>[2x]MATATEQWVLVEMVQALYEAPAYHLILEGILILWIIRLLFSKTYKLQERSDLTVKEKEELIEEWQPEPLVPPVPKDHPALNYNIVSGPPSHKTVVNGKECINFASFNFLGLLDNPRVKAAALASLKKYGVGTCGPRGFYGTFDVHLDLEDRLAKFMKTEEAIIYSYGFATIASAIPAYSKRGDIVFVDRAACFAIQKGLQASRSDIKLFKHNDMADLERLLKEQEIEDQKNPRKARVTRRFIVVEGLYMNTGTICPLPELVKLKYKYKARIFLEESLSFGVLGEHGRGVTEHYGINIDDIDLISANMENALASIGGFCCGRSFVIDHQRLSGQGYCFSASLPPLLAAAAIEALNIMEENPGIFAVLKEKCGQIHKALQGISGLKVVGESLSPAFHLQLEESTGSREQDVRLLQEIVDQCMNRSIALTQARYLEKEEKCLPPPSIRVVVTVEQTEEELERAASTIKEVAQAVLL;>MRPEPGGCCCRRTVR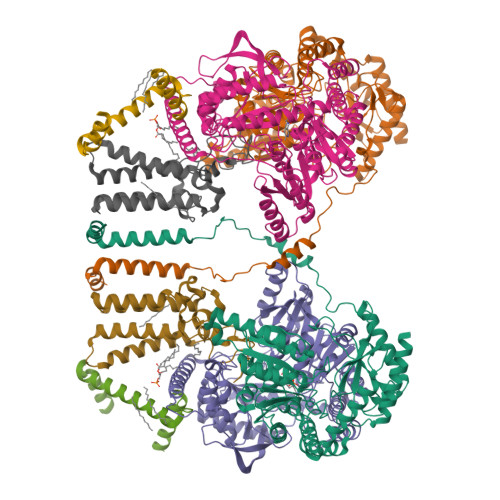ANGCVANGEVRNGYVRSSAAAAAAAAAGQIHHVTQNGGLYKRPFNEAFEETPMLVAVLTYVGYGVLTLFGYLRDFLRYWRIEKCHHATEREEQKDFVSLYQDFENFYTRNLYMRIRDNWNRPICSVPGARVDIMERQSHDYNWSFKYTGNIIKGVINMGSYNYLGFARNTGSCQEAAAKVLEEYGAGVCSTRQEIGNLDKHEELEELVARFLGVEAAMAYGMGFATNSMNIPALVGKGCLILSDELNHASLVLGARLSGATIRIFKHNNMQSLEKLLKDAIVYGQPRTRRPWKKILILVEGIYSMEGSIVRLPEVIALKKKYKAYLYLDEAHSIGALGPTGRGVVEYFGLDPEDVDVMMGTFTKSFGASGGYIGGKKELIDYLRTHSHSAVYATSLSPPVVEQIITSMKCIMGQDGTSLGKECVQQLAENTRYFRRRLKEMGFIIYGNEDSPVVPLMLYMPAKIGAFGREMLKRNIGVVVVGFPATPIIESRARFCLSAAHTKEILDTALKEIDEVGDLLQLKYSRHRL[2x];>[2x]MAGMALARAWKQMSWFYYQYLLVTALYMLEPWERTVFNSMLVSIVGMALYTGYVFMPQHIMAILHYFEIVQ;>[2x]MNVGTAHSEVNPNTRVMNSRGIWLSYVLAIGLLHIVLLSIPFVSVPVVWTLTNLIHNMGMYIFLHTVKGTPFETPDQGKARLLTHWEQMDYGVQFTASRKFLTITPIVLYFLTSFYTKYDQIHFVLNTVSLMSVLIPKLPQLHGVRIFGINKY> GAMESLPVIAAPSMWTRPQIKDFKEKIQQDADSVITVGRGEVVTVRVPTHEEGSYLFWEFATDNYDIGFGVYFEWTDSPNTAVSVHVSESSDDDEEEEENIGCEEKAKKNANKPLLDEIVP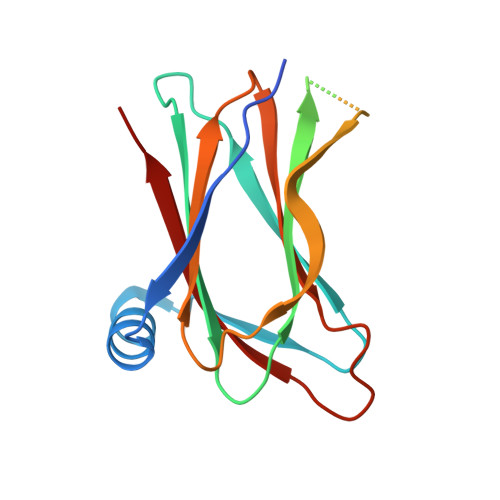VYRRDCHEEVYAGSHQYPGRGVYLLKFDNSYSLWRSKSVYYRVYYTR> LYEDPPDQKTSPSGKPATLKICSWNVDGLRAWIKKKGLDWVKEEAPDILCLQETKCSENKLPAELQELPGLSHQYWSAPSDKEGYSGVGLLSRQCPLKVSYGIGDEEHDQEGRVIVAEFDSFVLVTAYVPNAGRGLVRLEYRQRWDEAFRKFLKGLASRKPLVLCGDLNVAHEEIDLRNPKGNKKNAGFTPQERQGFGELLQAVPLADSFRHLYPNTPYAYTFWTYMMNARSKNVGWRLDYFLLSHSLLPA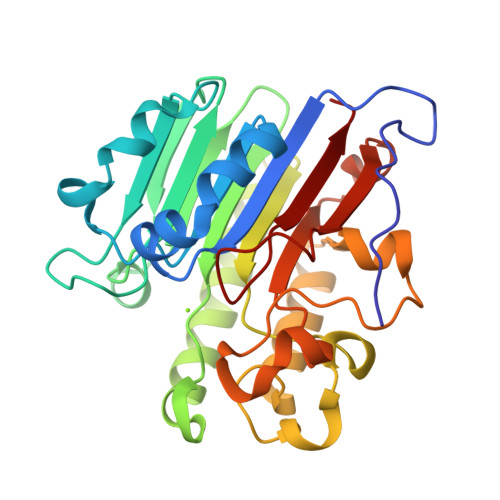LCDSKIRSKALGSDHCPITLYLAL7-(1~{H}-1,2,3-triazol-5-yl)quinazolin-2-amine | C10 H8 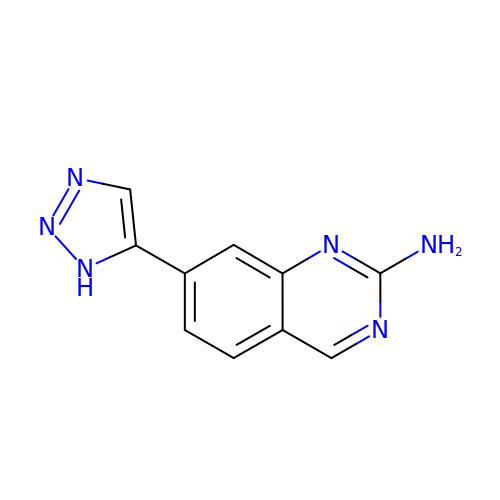N6 | BRODMNADNZNYMX-UHFFFAOYSA-N>[6x]HSYRIVVDPKEVVKPISRHIYGHFTEHLGRCIYGGIYEEGSPLSDERGFRKDVLEAVKRIKVPNLR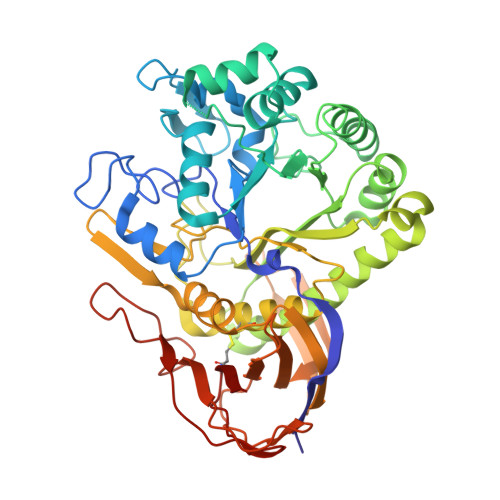WPGGNFVSNYHWEDGIGPKDQRPVRFDLAWQQEETNRFGTDEFIEYCREIGAEPYISINMGTGTLDEALHWLEYCNGKGNTYYAQLRRKYGHPEPYNVKFWGIGNEMYGEWQVGHMTADEYARAAKEYTKWMKVFDPTIKAIAVGCDDPIWNLRVLQEAGDVIDFISYHFYTGSDDYYETVSTVYLLKERLIGVKKLIDMVDTARKRGVKIALDEWNVWYRVSDNKLEEPYDLKDGIFACGVLVLLQKMSDIVPLANLAQLVNALGAIHTEKDGLILTPVYKAFELIVNHSGEKLVKTHVESETYNIEGVMFINKMPFSVENAPFLDAAASISEDGKKLFIAVVNYRKEDALKVPIRVEGLGQKKATVYTLTGPDVNARNTMENPNVVDITSETITVDTEFEHTFKPFSCSVIEVE> MNDDRETPPKRKPGEDDTLFDIDFLDDTTSHSGSRSKVTNSHANANYIPPSHVLPEETIDLDADDDNIENDVHENLFMSNNHDDQTSWNANRFDSDAYQPQSLRA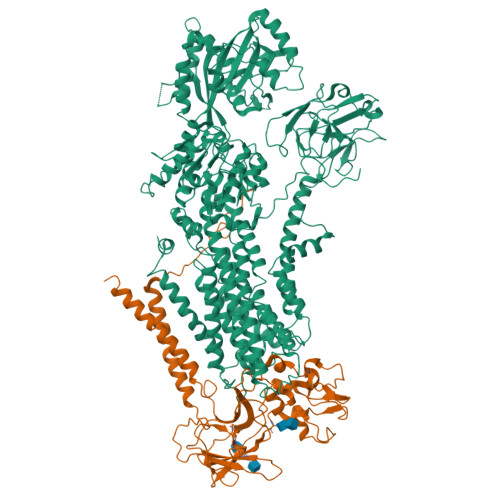VKPPGLFARFGNGLKNAFTFKRKKGPESFEMNHYNAVTNNELDDNYLDSRNKFNIKILFNRYILRKNVGDAEGNGEPRVIHINDSLANSSFGYSDNHISTTKYNFATFLPKFLFQEFSKYANLFFLCTSAIQQVPHVSPTNRYTTIGTLLVVLIVSAMKECIEDIKRANSDKELNNSTAEIFSEAHDDFVEKRWIDIRVGDIIRVKSEEPIPADTIILSSSEPEGLCYIETANLDGETNLKIKQSRVETAKFIDVKTLKNMNGKVVSEQPNSSLYTYEGTMTLNDRQIPLSPDQMILRGATLRNTAWIFGLVIFTGHETKLLRNATATPIKRTAVEKIINRQIIALFTVLIVLILISSIGNVIMSTADAKHLSYLYLEGTNKAGLFFKDFLTFWILFSNLVPISLFVTVELIKYYQAFMIGSDLDLYYEKTDTPTVVRTSSLVEELGQIEYIFSDKTGTLTRNIMEFKSCSIAGHCYIDKIPEDKTATVEDGIEVGYRKFDDLKKKLNDPSDEDSPIINDFLTLLATCHTVIPEFQSDGSIKYQAASPDEGALVQGGADLGYKFIIRKPNSVTVLLEETGEEKEYQLLNICEFNSTRKRMSAIFRFPDGSIKLFCKGADTVILERLDDEANQYVEATMRHLEDYASEGLRTLCLAMRDISEGEYEEWNSIYNEAATTLDNRAEKLDEAANLIEKNLILIGATAIEDKLQDGVPETIHTLQEAGIKIWVLTGDRQETAINIGMSCRLLSEDMNLLIINEETRDDTERNLLEKINALNEHQLSTHDMNTLALVIDGKSLGFALEPELEDYLLTVAKLCKAVICCRVSPLQKALVVKMVKRKSSSLLLAIGDGANDVSMIQAAHVGVGISGMEGMQAARSADIAVGQFKFLKKLLLVHGSWSYQRISVAILYSFYKNTALYMTQFWYVFANAFSGQSIMESWTMSFYNLFFTVWPPFVIGVFDQFVSSRLLERYPQLYKLGQKGQFFSVYIFWGWIINGFFHSAIVFIGTILIYRYGFALNMHGELADHWSWGVTVYTTSVIIVLGKAALVTNQWTKFTLIAIPGSLLFWLIFFPIYASIFPHANISREYYGVVKHTYGSGVFWLTLIVLPIFALVRDFLWKYYKRMYEPETYHVIQEMQKYNISDSRPHVQQFQNAIRKVRQVQRMKKQRGFAFSQAEEGGQEKIVRMYDTTQKRGKYGELQDASANPFNDNNGLGSNDFESAEPFIENPFADGNQNSNRFSSSRDDISFDI;> MVSLFKRGKAPPLTKEGPTSKKPPNTAFRQQRLKAWQPILSPQSVLPLLIFVACIFTPIGIGLIVSATKVQDLTIDYSHCDTKASTTAFEDIPKKYIKYHFKSKVENKPQWRLTENENGEQSCELQFEIPNDIKKSIFIYYKITNFYQNHRRYVQSFDTKQILGEPIKKDDLDTSCSPIRSREDKIIYPCGLIANSMFNDTFSQVLSGIDDTEDYNLTNKHISWSIDRHRFKTTKYNASDIVPPPNWMKKYPDGYTDENLPDIHTWEEFQVWMRTAAFPKFYKLTLKNESASLPKGKYQMNIELNYPISLFGGTKSFVLTTNGAIGGRNMSLGVLYLIVAGLCALFGIIFLVKLIFQPRAMGDHTYLNFDDEENEDYEDVHAENTTLREIL>GSARKEEEGTTIEKLLNEMQELLTLTDSDKIKELSLKNSGLLEQHDPTLAMFGNMPKGEIVALISSLLQSKFVKIELKKKYAKLLLDLLGEDDWELALLSWLGVGELNQEGIQKIKKLYEKAKDEDSENGASLLDWFMEIKDLPEREKHLKVIIRALSFDLSYMSSFEDKVRTSSIISDLCRIIIFLSLNNYTDIIAISIKKDKDVILNEMLSIIEHVWLTED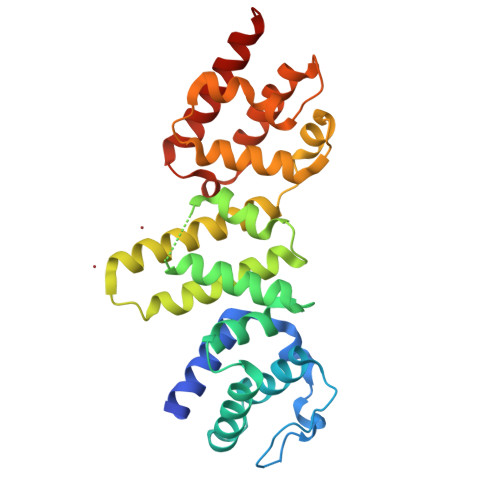WLLESPSRVSIVEDKHVYYFHLLKEFFASLPDACFIDNEQRSNTLLMIGKVIDYKEDVM[2x]> TLRTVADLMSDKEKVRHN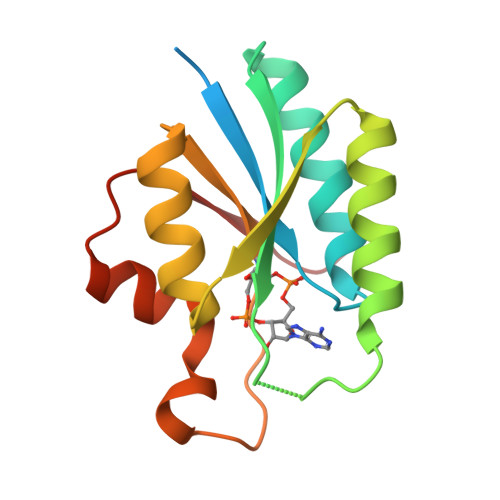HKTSLKPHIAVAISGSIYNEAVIKEAFHIAQKEHAKFTAIYIDVFEKSRQYKDSQKQVHQHLMLAKSLGAKVKVVYSQTVALGLDEWCKNQDVTKLIIGQHIRNKRRDFFNKPLIDHLMSFEHSYKIEIVPIKQ> MTLKVILGEHQITRTELLVGIATVSGCGAVVYCISKFWGYGAIAPYPQSGGNRVTRALQRAVIDKTKTPIETRFYPLDSLRTVTPKRVADNGHAVSGAVRDAARRLIDESITAVGGSKFEVNPNPNSSTGLRNHFHFAVGD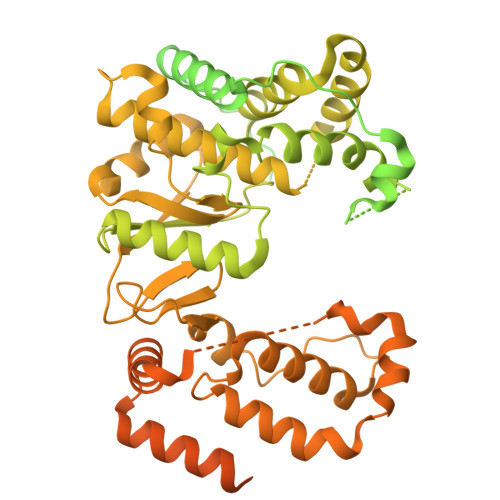LAQDFRNDTPADDAFIVGVDVDYYVTEPDVLLEHMRPVVLHTFNPKKVSGFDADSPFTIKNNLVEYKVSGGAAWVHPVWDWCEAGEFIASRVRTSWKEWFLQLPLRMIGLEKVGYHKIHHCRPWTDCPDRALVYTIPQYVIWRFNWIDTELHVRKLKRIEYQDETKPGWNRLEYVTDKNELLVSIGREGEHAQITIEKEKLDMLSGLSATQSVNARLIGMGHKDPQYTSMIVQYYTGKKVVSPISPTVYKPTMPRVHWPVTSDADVPEVSARQYTLPIVSDCMMMPMIKRWETMSESIERRVTFVANDKKPSDRIAKIAETFVKLMNGPFKDLDPLSIEETIERLNKPSQQLQLRAVFEMIGVKPRQLIESFNKNEPGMKSSRIISGFPDILFILKVSRYTLAYSDIVLHAEHNEHWYYPGRNPTEIADGVCEFVSDCDAEVIETDFSNLDGRVSSWMQRNIAQKAMVQAFRPEYRDEIISFMDTIINCPAKAKRFGFRYEPGVGVKSGSPTTTPHNTQYNGCVEFTALTFEHPDAEPEDLFRLIGPKCGDDGLSRAIIQKSINRAAKCFGLELKVERYNPEIGLCFLSRVFVDPLATTTTIQDPLRTLRKLHLTTRDPTIPLADAACDRVEGYLCTDALTPLISDYCKMVLRLYGPTASTEQVRNQRRSRNKEKPYWLTCDGSWPQHPQDAHLMKQVLIKRTAIDEDQVDALIGRFAAMKDVWEKITHDSEESAAACTFDEDGVAPNSVDESLPLLNDAKQTRANPGTSRPHSNGGGSSHGNELPRRTEQRAQGPRQPARLPKQGKTNGKSDGNITAGETQRGGIPRGKGPRGGKTNTRRTPPKAGAQPQPSNNRKSRLEEELRRRLTE>[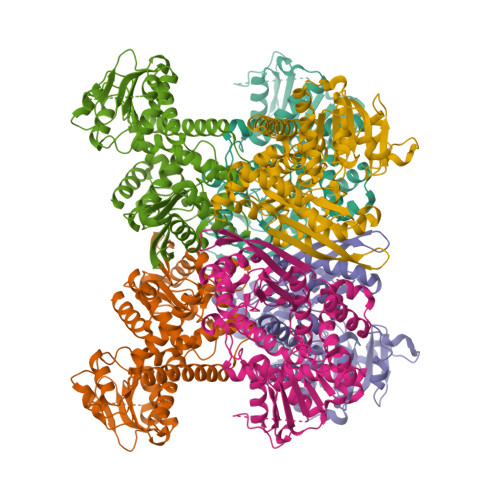6x]MAADRNTGHTEEDKLDVLKSTQTVIHKALEKLGYPEEVYELLKEPMRLLTVKIPVRMDDGSVKIFTGYRAHNDSVGPTKGGIRFHPNVTEKEVKALSIWMSLKCGIIDLPYGGGKGGIVCDPRDMSFRELERLSRGYVRAISQIVGPTKDVPAPDVFTNSQIMAWMMDEYSRIDEFNSPGFITGKPLVLGGSHGRESATAKGVTICIKEAAKKRGIDIKGARVVVQGFGNAGSYLAKFMHDAGAKVVGISDAYGGLYDPEGLDIDYLLDRRDSFGTVTKLFNDTITNQELLELDCDILVPAAIENQITEENAHNIRAKIVVEAANGPTTLEGTKILSDRDILLVPDVLASAGGVTVSYFEWVQNNQGFYWSEEEVEEKLEKMMVKSFNNIYEMANNRRIDMRLAAYMVGVRKMAEASRFRGWI> MQLTPTFYDNSCPNVSNIVRDTIVNELRSDPRIAASILRLHFHDCFVNGCDASILLDNTTSFRTEKDAFGNANSARGFPVIDRMKAAVESACPRTVSCADLLTIAAQQSVTLAGGPSWRVPLGRRDSLQAFLDLAN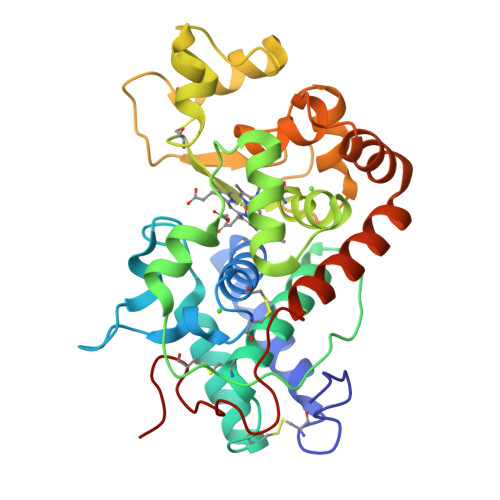ANLPQPFFTLPQLKDSFRNVGLNRSSDLVALSGGHTFGKNQCRFIMDRLYNFSNTGLPDPTLNTTYLQTLRGLCPLNGNLSALVDFDLRTPTIFDNKYYVNLEEQKGLIQSDQELFSSPNATDTIPLVRSFANSTQTFFNAFVEAMDRMGNITPLTGTQGQIRLNCRVVNSNS> NLRVLLDTAIPPSFCDTVSSVLLDDFNMVSLIRTSPADSLATIKQDNAEIDIAITIDEELKISRFNQCVLGYTKAFVVAHPQHPLCNASLHSIASLANYRQISLGSRSGQHSNLLRPVSDKVLFVENFDDMLRLVEAGVGWGIAPHYFVEERLRNGTLAVLSELYEPGGIDTKVYCYYNTALESERSFLRFLESARQRLRELGRQRFDDAPAWQPS

PA possesses three QS systems known as las, rhl, and the Pseudomonas Quinolone System (pqs). The biosynthesis of AQs including the signal molecules 2-heptyl-3-hydroxy-4(1H)-quinolone (PQS) and 2-heptyl-4-hydroxyquinoline (HHQ) depends on a group of enzymes (PqsA, PqsBC, PqsD, PqsE, PqsH) and the starting substrates, anthraniloyl-CoA and malonyl-CoA. Both PQS, and HHQ bind to the LysR type regulator PqsR (also called MvfR) inducing conformational changes and leading to a positive feedback loop through the transcriptional activation of the pqsABCDE operon. PqsR was therefore identified as a critical element for a fully functional pqs system. X-ray crystallography techniques were employed in this study to gain a deeper understanding of the conformation and binding interactions of this series of inhibitors within the PqsR coinducer binding domain using crystal soaking experiments under the conditions reported by Soukarieh et al. Several reports noted that the PqsR receptor ligand binding domain consists of two subdomains known as pocket A (deep slot) and B (outer pocket) connected by an antiparallel β sheet hinge region.

To enhance the physiochemical properties of the series through reducing lipophilicity, analogues with polar substituents were synthesized (6t R3 = methoxyethyl, 6u R3 = hydroxyethyl, and 6q R3 = dimethylaminoethyl). Compounds 6t and 6u were equipotent in PAO1-L with a 2-fold reduction in potency in relation to 6f, however, a structurally related dimethylamino-ethyl substitution in 6q obliterated the biological activity. To achieve this aim, two crystal structures of inhibitors (6f and 6t) complexed with the PqsRLBD were obtained. These revealed that both compounds bind in a similar manner to our previously reported PqsR inhibitor 1(25) except for an additional interaction between the 2-amino group and Arg209, which may have contributed to the enhancement of activity noted for the current series of compounds. The para-phenyl acetonitrile group of 6f, 6t adopted a parallel position to the Tyr258 in pocket B to maintain hydrophobic interactions as the case in 1. While the hydroxyl group position was altered slightly between the two series leading to form hydrogen bond with Leu208 and Arg209 in the benzimidazole derivatives compared to Leu208 and Glu194 in the quinazolinone derived inhibitor. However, unlike 1,136f and 6t form an additional hydrogen bond between the amino group at the 2-postion of the benzimidazole ring and the backbone of of Leu207, which may contribute to the observed enhanced potency. The crystal structure also corroborated our rational design that the lipophilic subpocket around (Leu207, Leu208, Ile236, and Ile263) can be exploited with lipophilic substituent at position 1 of the benzimidazole ring.> GHMTIARDIVLQESIGKGRFGEVWRGKWRGEEVAVKIFSSREERSWFREAEIYQTVMLRHENILGFIAADNKDNGTWTQLWLVSDYHEHGSLFDYLNRYTVTVEGMIKLALSTASGLAHLHMEIVGTQGK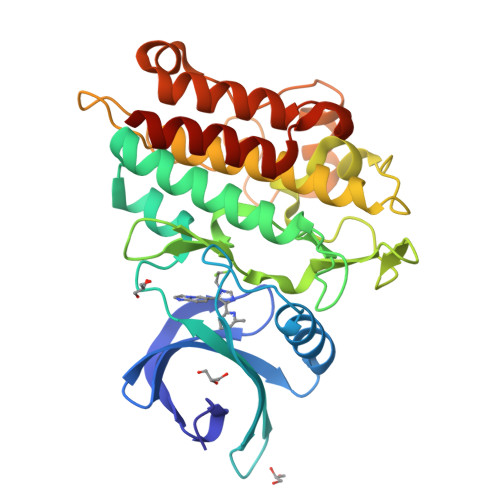PAIAHRDLKSKNILVKKNGTCCIADLGLAVRHDSATDTIDIAPNHRVGTKRYMAPEVLDDSINMKHFESFKRADIYAMGLVFWEIARRCSIGGIHEDYQLPYYDLVPSDPSVEEMRKVVCEQKLRPNIPNRWQSCEALRVMAKIMRECWYANGAARLTALRIKKTLSQLSQQEGIKM4-amino-N-(pyridin-2-yl)benzenesulfonamide | C11 H11 N3 O2 S | 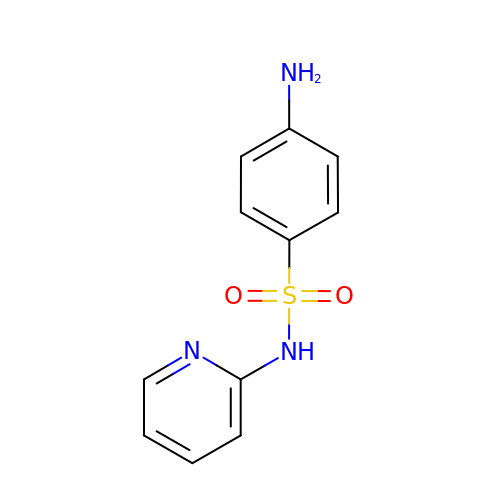GECHUMIMRBOMGK-UHFFFAOYSA-N6-azanyl-9-[(3~{R})-1-[(~{E})-but-2-enoyl]pyrrolidin-3-yl]-7-(4-phenoxyphenyl)purin-8-one 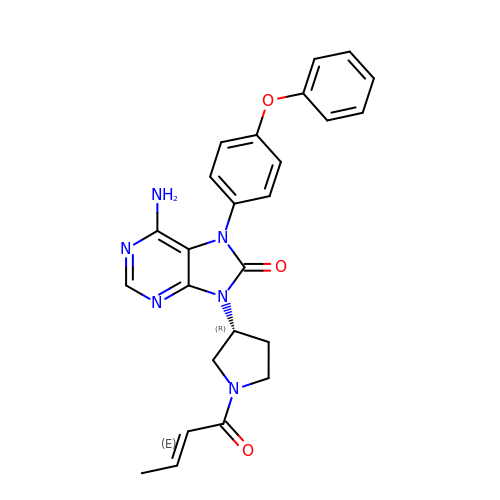| C25 H24 N6 O3 | ZHAZXTKPNSTGRP-OBNPVOHOSA-N3-[5-{[3-(2-carboxyethyl)-4-(carboxymethyl)-5-methyl-1H-pyrrol-2-yl]methyl}-4-(carboxymethyl)-1H-pyrrol-3-yl]propanoic acid | C20 H24 N2 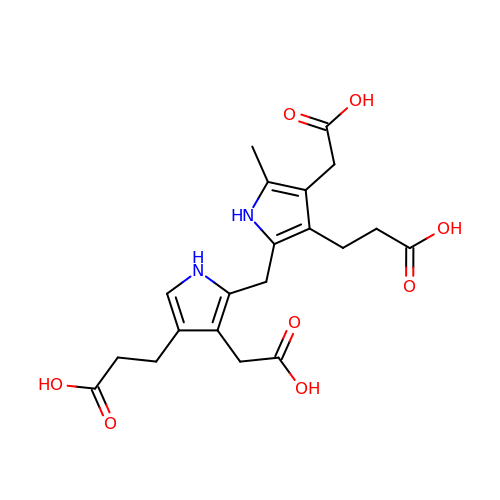O8 | LCAXMKQKEYTFDM-UHFFFAOYSA-N>SNAMKWKKSLAGLSSYKPGKREEEVMAELGLTKITKLSSNENPLGTSKKVAAIQANSSVETEIYPDGWASSLRKEVADFYQLEEEELIFTAGVDELIELLTRVLLDTTTNTVMATPTFVQYRQNALIEGAEVREIPLLQDGEHDLEGMLNAIDEKTTIVWICNPNNPTGNYIELADIQAFLDRVPSDVLVVLDEAYIEYVT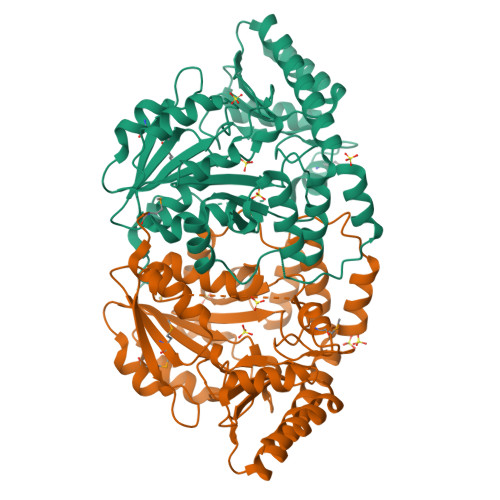PQPEKHEKLVRTYKNLIITRTFSKIYGLASARVGYGIADKEIIRQLNIVRPPFNTTSIGQKLAIEAIKDQAFIGECRTSNANGIKQYEAFAKRFEKVKLYPANGNFVLIDLGIEAGTIFSYLEKNGYITRSGAALGFPTAVRITIGKEEDNSAVIALLEKLL[2x]> MIFSVDKVRADFPVLSREVNGLPLAYLDSAASAQKPSQVIDAEAEFYRHGYAAVHRGIHTLSAQATEKMENVRKRASLFINAR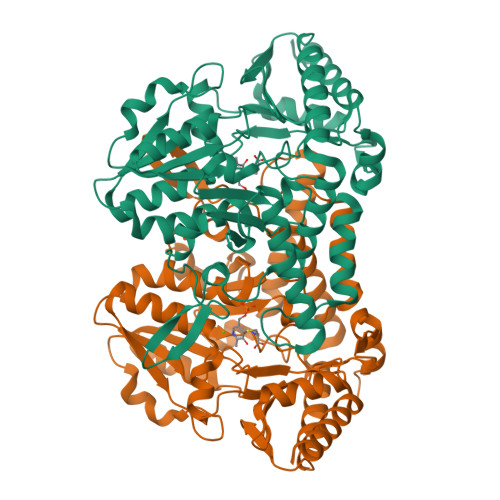SAEELVFVRGTTEGINLVANSWGNSNVRAGDNIIISQMEHHANIVPWQMLCARVGAELRVIPLNPDGTLQLETLPTLFDEKTRLLAITHVSNVLGTENPLAEMITLAHQHGAKVLVDGAQAVMHHPVDVQALDCDFYVFSGHKLYGPTGIGILYVKEALLQEMPPWEGGGSMIATVSLSEGTTWTKAPWRFEAGTPNTGGIIGLGAALEYVSALGLNNIAEYEQNLMHYALSQLESVPDLTLYGPQNRLGVIAFNLGKHHAYDVGSFLDNYGIAVRTGHHAAMPLMAYYNVPAMCRASLAMYNTHEEVDRLVTGLQRIHRLLG>[8x]DNKELKIIRKDVAECLRTLPKCGNQPDDPLARVDVWHCAMAKRGVYDNPDPAVIKERSM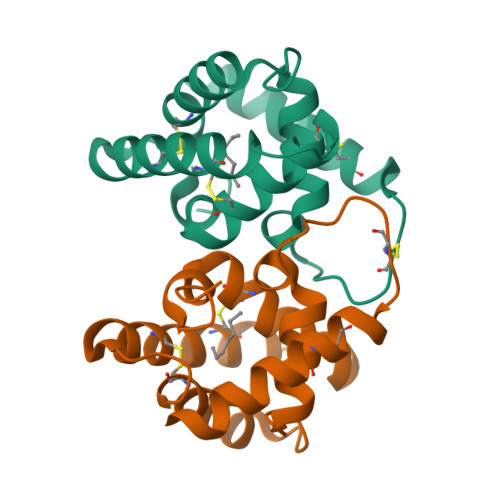KMCTKIITDPANVENCKKVASRCVDRETQGPKSNRQKAVNIIGCALRAGVAETTVLARKKHHHHHH>[2x]IVGGTNASLGEWPWQVSLQVKLVSQTHLCGGSIIGRQWVLTAAHCFDGIPYPDV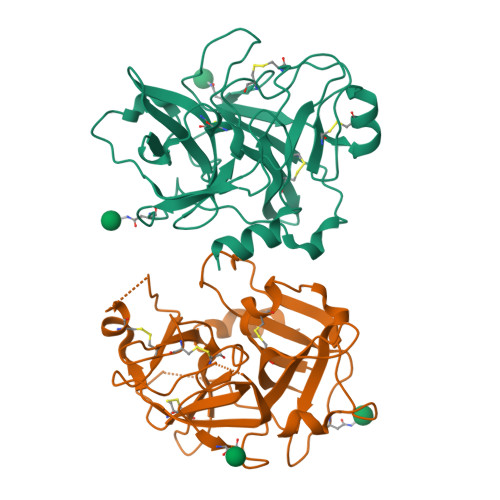WRIYGGILSLSEITKETPSSRIKELIIHQEYKVSEGNYDIALIKLQTPLNYTEFQKPISLPSKADTNTIYTNCWVTGWGYTKEQGETQNILQKATIPLVPNEECQKKYRDYVINKQMICAGYKEGGTDACKGDSGGPLVCKHSGRWQLVGITSWGEGCARKDQPGVYTKVSEYMDWILEKTQSSDVRALETSSAVD>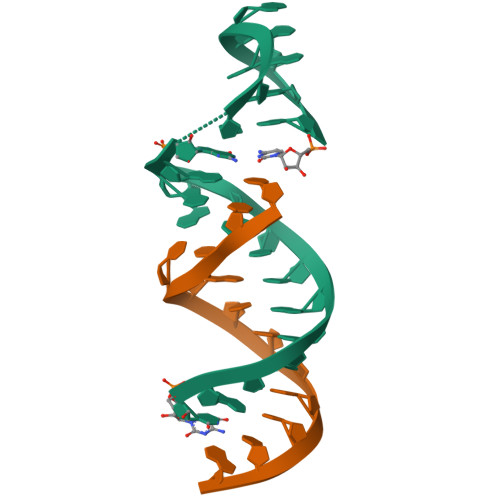 XUGCUGGCUAAGGXCCGAAAGG;> CUAUGCCUGCUG>[4x]MHFETTKDGFTIAIGNRIILSHSPDKPAFFAGFGEERMDMYRGNFDIEDYVIERTALRHAEVSGDSVTLSSAPGQAPRLRLTLDGNAIRLTALDETINRLWLRVVAETDEHVWGGGEQMSYFDMRGRRFPLWTSEPGVGRDKTTEITFKSDVSGKAGGDYYNTNYPQPTWLSSRKYALHVETSAYSVFDFRNGDFHEIEIWAVPEKIEFFAGDSFADIVSALSLHFGRQPELPDWVYNGAIIGLKDGVNSFARLEKIRAAGTKVSGLWCEDWVGLRQTSFGARLFWDWQANDTRYPHLRQKIAELADQGIRFLGYVNPYLCVDGPLFPVAESAGYFATDVDGKTALVDFGEFDCGVVDFTNPAAADWFAAAIIGKNMLDFGLSGWMADFGEYLPIDIKLSNGVDAKLMHNAWPTLWAEVNAKGVESRGKTGEALFFMRAGFTGVQAHCPLIWGGNQSVDFSRHDGLVTVICGALSSGLMGNAYHHSDIGGYT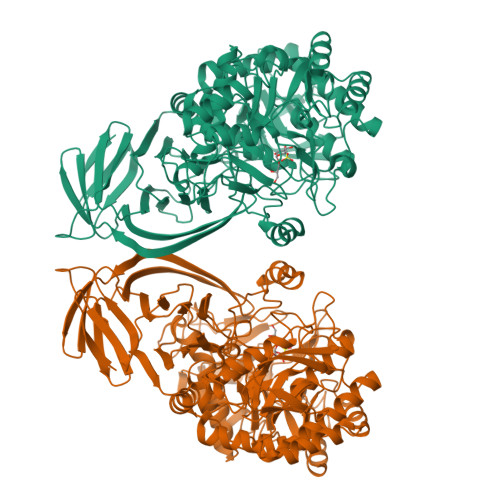SLFGNVRTAELIMRWTEMAAFTPVMRTHEGNRPRDNLQIDQDETVLAHFARMTAIYVALAPYLKSLSAEAAKTGLPVQRPLFLHYENEPQTYAVQDCYLYGADMLVAPVWKAGETQRSLYLPGHGEWVHLWSGKRHAGGRDITVETPLGEPAVFYRADSSHHRLFEQLRTIGLEHHHHHH In most bacteria, iron homeostasis is regulated primarily by the ferric uptake regulator (Fur). Fur, which was first discovered in Escherichia coli, is a global transcriptional regulator that directly controls the transcription of over 90 genes involved in iron uptake, storage and metabolism. Several holo-Fur structures have been solved, revealing a modular domain organization including an N-terminal DNA-binding domain (DBD) and a C-terminal dimerization domain (DD). In this study, we present six crystal structures of apo-Fur, holo-Fur, Fur in complex with the Fe2+ transport protein (feoAB1) operator and the P. aeruginosa (or E. coli) Fur box.

We produced a C9L/M14L/M16V-triple mutant that successfully generated diffraction-quality holo-Fur crystals. The overall structure of holo-Fur was a homodimer with the same secondary structure as that of apo-Fur. The two monomers in holo-Fur had nearly identical conformations (r.m.s.d.=0.36 Å) that differed substantially from those in apo-Fur. The large difference between the apo- and holo-Fur structures arose from the conformations of the two N-terminal DBDs and two hinges. Thus, the binding of two Mn2+ ions stabilized the hinge conformation and induced profound conformational changes of the DBD. Each holo-Fur monomer contains two Mn2+-binding sites (site 1 and site 2). Site 1 links the DBD and DD. This site contains a manganese ion, Mn1, that is hexacoordinated by two residues (H33 and E81) from the DBD and three residues (H88, H90 and E101) from the DD. Site 2 resides almost entirely in the DD, within the β3 and β5 strands and α5 helix. In site 2, the manganese ion, Mn2, is also hexacoordinated by residues H87, D89, E108, H125 and Q111, while a water molecule mediates interactions with the latter.

>[2x]GHMVSRIEQRLIDKGLKVTDQRRVIAQVLSDSADHPDVEEVYRRATAKDPRISIATVYRTVRLFEEESILERHDFGDGRARYEEAPSEHHDHLIDVNSARVIEFTSPEIEALQREIARKHGFRLVGHRLELYGVPLTSGGDSDDK>[2x]MPHFTVVPVDGPRRGDYDNLEGLSWVDYGERAELDDSDGHGNHRESSPFLSPLEASRGIDYYDRNLALFEEELDIRPKVSSLLGKLVSYTNLTQGAKEHEEAESGEGTRRRAAEAPSMGTLMGVYLPCLQNIFGVILFLRLTWMVGTAGVLQALLIVLICCCCTLLTAISMSAIATNGVVPAGGSYFMISRSLGPEFGGAVGLCFYLGTTFAAAMYILGAIEILLTYIAPPAAIFYPSGAHDTSNATLNNMRVYGTIFLTFMTLVVFVGVKYVNKFASLFLACVIISILSIYAGGIKSIFDPPVFPVCMLGNRTLSRDQFDICAKTAVVDNETVATQLWSFFCHSPNLTTDSCDPYFMLNNVTEIPGIPGAAAGVLQENLWSAYLEKGDIVEKHGLPSADAPSLKESLPLYVVADIATSFTVLVGIFFPSVTGIMAGSNRSGDLRDAQKSIPVGTILAIITTSLVYFSSVVLFGACIEGVVLRDKYGDGVSRNLVVGTLAWPSPWVIVIGSFFSTCGAGLQSLTGAPRLLQAIAKDNIIPFLRVFGHGKVNGEPTWALLLTALIAELGILIASLDMVAPILSMFFLMCYLFVNLACAVQTLLRTPNWRPRFKYYHWALSFLGMSLCLALMFVSSWYYALVAMLIAGMIYKYIEYQGAEKEWGDGIRGLSLSAARYALLRLEEGPPHTKNWRPQLLVLLKLDEDLHVKYPRLLTFASQLKAGKGLTIVGSVIQGSFLESYGEAQAAEQTIKNMMEIEKVKGFCQVVVASKVREGLAHLIQSCGLGGMRHNSVVLGWPYGWRQSEDPRAWKTFIDTVRCTTAAHLALLVPKNIAFYPSNHERYLEGHIDVWWIVHDGGMLMLLPFLLRQHKVWRKCRMRIFTVAQMDDNSIQMKKDLAVFLYHLRLEAEVEVVEMHNSDISAYTYERTLMMEQRSQMLRQMRLTKTEREREAQLVKDRHSALRLESLYSDEE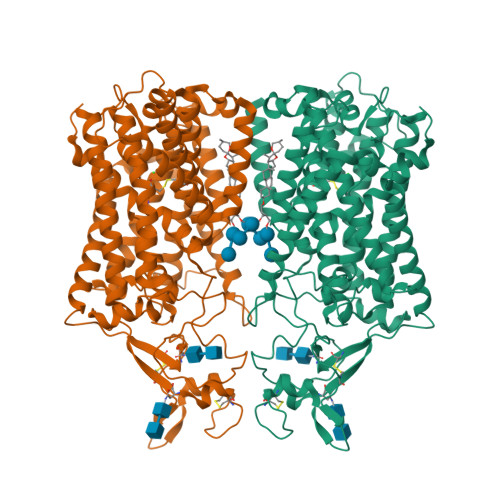DESAVGADKIQMTWTRDKYMTETWDPSHAPDNFRELVHIKPDQSNVRRMHTAVKLNEVIVTRSHDARLVLLNMPGPPRNSEGDENYMEFLEVLTEGLERVLLVRGGGREVITIYSLEWSHPQFEK> MSTAKVTLVTSGGSSQDFTSEQTNITTDFARVRVTKGMWIFYQQANYNDASGGGSLWIKLDESSHLMDLPFTPRSFRPVKTFQVGATLYKHVNFGGKELDLPNS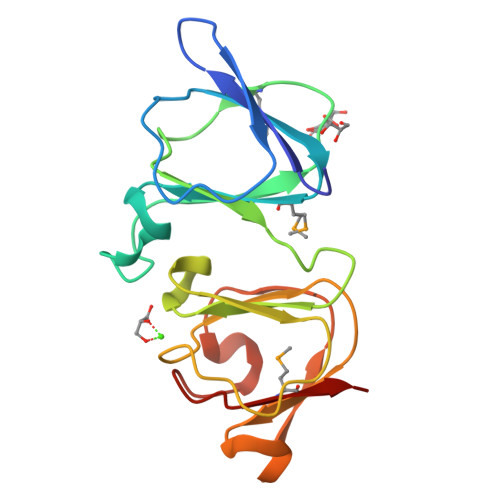NPRIDIGGVSSALISQGQWRLYEQYDYAGPSTRRGPGVYVNAGALGVANDALKSMEREF N'-[(3S,4R,5S,8R,9E,12S,14S,15R,16S,18R,19R,26aS)-5,19-dihydroxy-3-{(1E)-1-[(1R,3R,4R)-4-hydroxy-3-methoxycyclohexyl]prop-1-en-2-yl}-14,16-dimethoxy-4,10,12,18-tetramethyl-1,20,21-trioxo-8-(prop-2-en-1-yl)-1,3,4,5,6,8,11,12,13,14,15,16,17,18,19,20,21,23,24,25,26,26a-docosahydro-7H-15,19-epoxypyrido[2,1-c][1,4]oxazacyclotricosin-7-ylidene]acetohydrazide 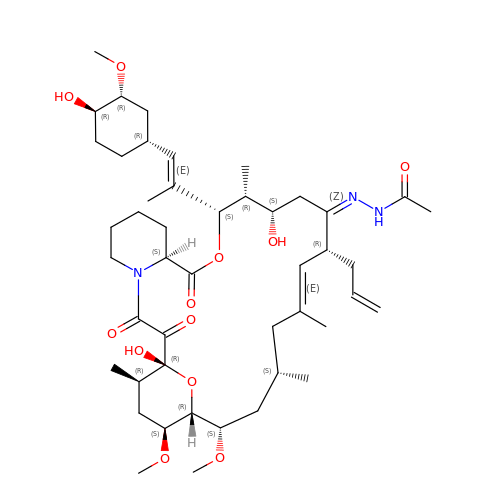| C46 H73 N3 O12 | SNUGJLTYIQECPY-OZIGKTPASA-N> MAFLMHLLVCVFGMGSWVTINGLWVELPLLVMELPEGWYLPSYLTVVIQLANIGPLLVTLLHHFRPSCLSEVPIIFTLLGVGTVTCIIFAFLWNMTSWVLDGHHSIAFLVLTFFLALVDCTSSVTFLPFMSRLPTYYLTTFFVGEGLSGLLPALVALAQGSGLTTCVNVTEISDSVPSPVPTRETDIAQGVPRALVSALPGMEAPLSHLESRYLPAHFSPLVFFLLLSIMMACCLVAFFVLQRQPRCWEASVEDLLNDQVTLHSIRPREENDLGPAGTVDSSQGQGYLEEKAAPCCPAHLAFIYTLVAFVNALTNGMLPSVQTYSCLSYGPVAYHLAATLSIVANPLASLVSMFLPNRSLLFLGVLS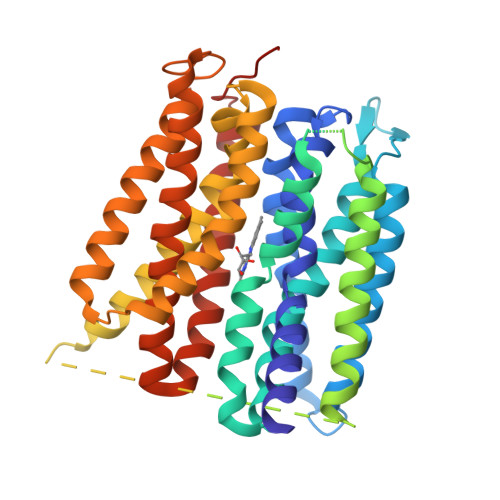VLGTCFGGYNMAMAVMSPCPLLQGHWGGEVLIVASWVLFSGCLSYVKVMLGVVLRDLSRSALLWCGAAVQLGSLLGALLMFPLVNVLRLFSSADFCNLHCPA>AEVNDPRVGFVAVVTFPVDGPATQHKLVELATGGVQEWIREVPGFLSATYHASTDGTAVVNYAQWESEQAYRVNFGADPRSAELREALSSLPG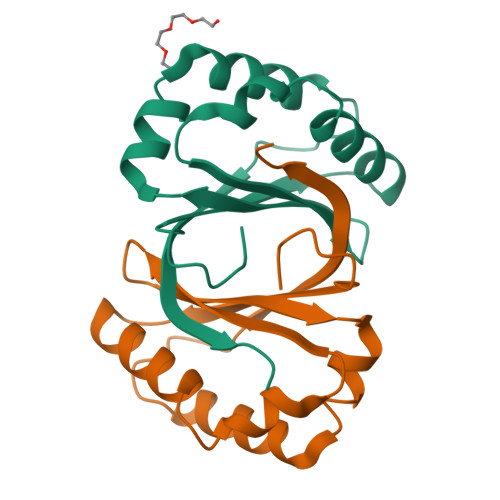LMGPPKAVFMTPRGAILPS[2x]> KL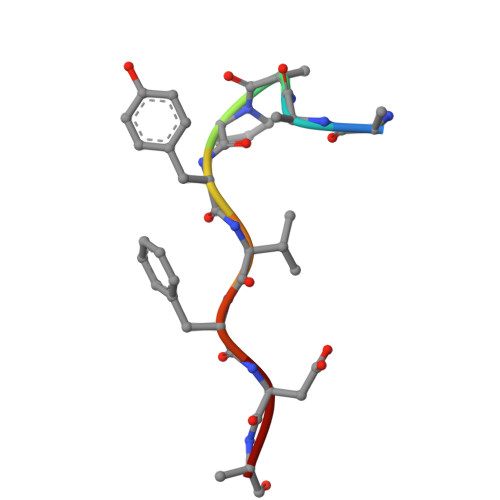KPYVFDY~{N}-[(3~{S})-pyrrolidin-3-yl]isoquinoline-5-sulfonamide | C13 H15 N3 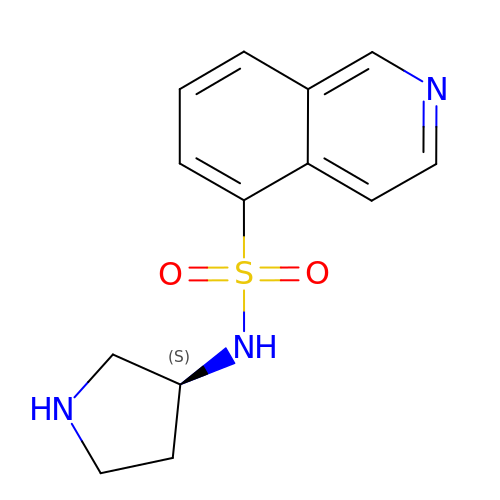O2 S | DPOHKNPOBZVTBK-NSHDSACASA-N> DNGGYVPAVVIGTGYGAAVSALRLGEAGVQTLMLEMGQLWNQPGPDGNIFCGMLNPDKRSSWFKNRTEAPLGSFLWLDVVNRNIDPYAGVLDRVNYDQMSVYVGRGVGGGSLVNGGMAVEPKRSYFEEILPRVDSSEMYDRYFPRANSMLRVNHIDTKWFEDTEWYKFARVSREQAGKAGLGTVFVPNVYDFGYMQREAAGEVPKSALATEVIYGNNHGKQSLDKTYLAAALGTGKVTIQTLHQVKTIRQTKDGGYALTVEQKDTDGKLLATKEISCRYLFLGAGSLGSTELLVRARDTGTLPNLNSEVGAGWGPNGNIMTARANHMWNPTGAHQ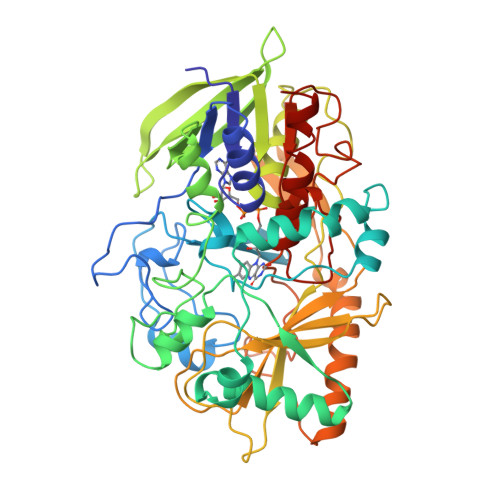SSIPALGIDAWDNSDSSVFAQIAPMPAGLETWVSLYLAITKNPQRGTFVYDAATDRAKLNWTRDQNAPAVNAAKALFDRINKANGTIYRYDLFGTQLKAFADDFCYHPLGGCVLGKATDDYGRVAGYKNLYVTDGSLIPGSVGVNPFVTITALAERNVERIIKQDVTAS4-{[6-(cyclohexylmethyl)pyridine-2-carbonyl]amino}-3-(phenylamino)benzoic 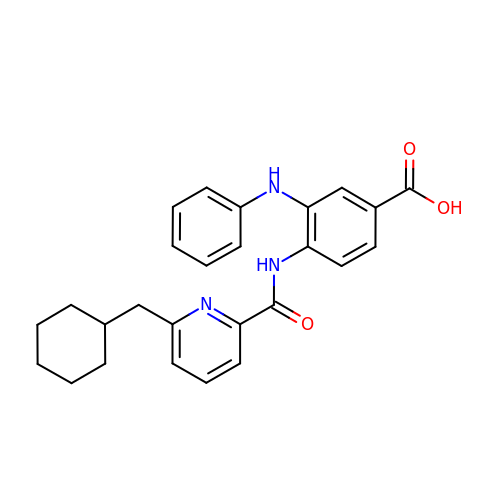acid | C26 H27 N3 O3 | PIPBPJWDZSBLMQ-UHFFFAOYSA-N> QECTKFKVSSCRECIESGPGCTWCQKLNFTGPGDPDSIRCDTRPQLLMRGCAADDIMDPTSLAETQEDHNGGQKQLSPQKVTLYLRPGQAAAFNVTFRRAKGYPIDLYYLM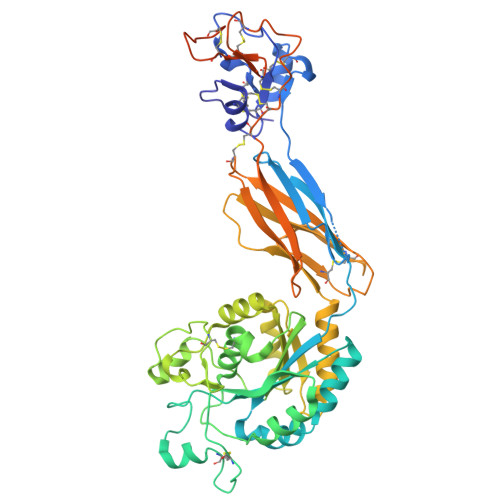DLSYSMLDDLRNVKKLGGDLLRALNEITESGRIGFGSFVDKTVLPFVNTHPDKLRNPCPNKEKECQPPFAFRHVLKLTNNSNQFQTEVGKQLISGNLDAPEGGLDAMMQVAACPEEIGWRKVTRLLVFATDDGFHFAGDGKLGAILTPNDGRCHLEDNLYKRSNEFDYPSVGQLAHKLAENNIQPIFAVTSRMVKTYEKLTEIIPKSAVGELSEDSSNVVQLIKNAYNKLSSRVFLDHNALPDTLKVTYDSFCSNGVTHRNQPRGDCDGVQINVPITFQVKVTATECIQEQSFVIRALGFTDIVTVQVLPQCECRCRDQSRDRSLCHGKGFLECGICRCDTGYIGKNCEPAALQTLFQGPLGAQGKKKLQALKKKNAQLKWKLQALKKKLAQHHHHHHA> MGSVGRVTAPEPLSAFHQVAEFVSGEAVLDDWLKQKGLKNQALGAARTFVVCKKDTKQVAGFYSLATGSV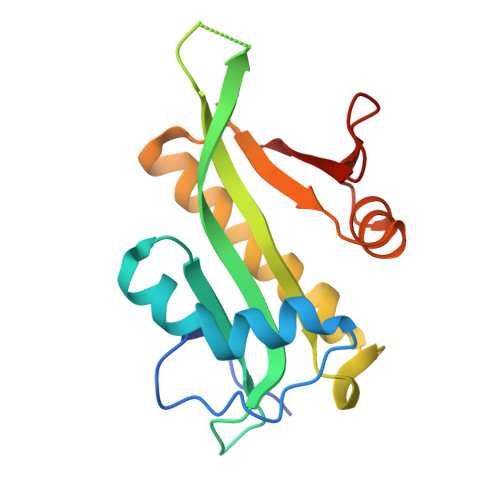NHTEATGNLRRNMPDPIPVIILARLAVDLSFHGKGLGADLLHDAVLRCYRVAENIGVRAIMVHALTEEAKNFFIHHGFKSSQTQQRTLFLRLPQ>[2x]MKTIGLLGGMSWESTIPYYRLINEGIKQRLGGLHSAQVLLHSVDFHEIEECQRRGEWDKTGDILAEAALGLQRAGAEGIVLCT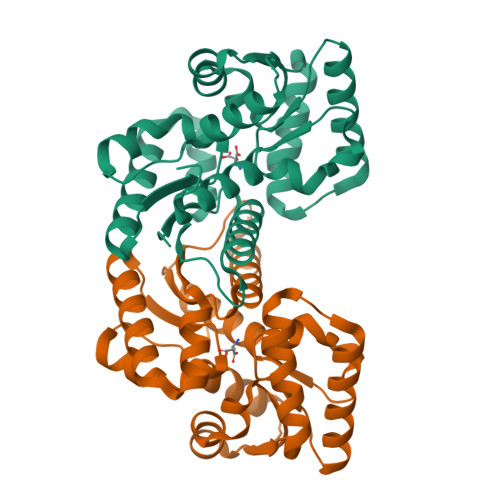NTMHKVADAIESRCTLPFLHIADATGRAITGAGMTRVALLGTRYTMEQDFYRGRLTEQFSINCLIPEADERAKINQIIFEELCLGQFTEASRAYYAQVIARLAEQGAQGVIFGCTEIGLLVPEERSVLPVFDTAAIHAEDAVAFMLSLEHHH> MVNAIRTPDQRFSNLDQYPFSPNYLDDLPGYPGLRAHYLDEGNSDAEDVFLCLHGEPTWSYLYRKMIPVFAESGARVIAPDFFGFGKSDKPVDEEDYTFEF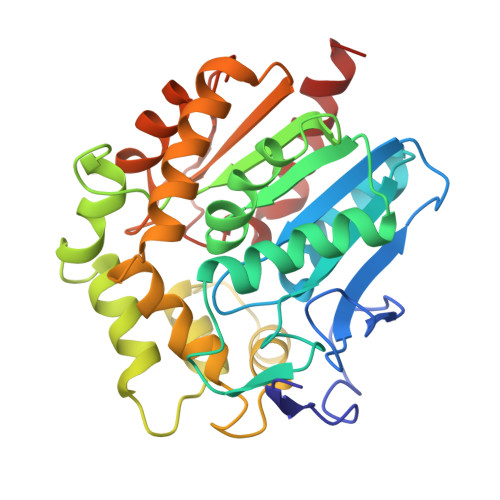HRNFLLALIERLDLRNITLVVQDWGGFLGLTLPMADPSRFKRLIIMNACLMTDPVTQPAFSAFVTQPADGFTAYKYDLVTPSDLRLDQFMKRWAPTLTEAEASAYAAPFPDTSYQAGVRKFPKMVAQRDQACIDISTEAISFWQNDWNGQTFMAIGMKDKLLGPDVMYPMKALINGCPEPLEIADAGHFVQEFGEQVAREALKHFAETE>[2x]MRGSHHHHHHGSGTDITNQLTNVTVGIDSGTTVYPHQAGYVKLNYGFSVPNSAVKGDTFKITVPKELNLNGVTSTAKVPPIMAGDQVLANGVIDSDGNVIYTFTDYVNTKCDVKATLTMPAYIDPENVKKTGNVTLATGIGSTTANKTVLVDYEKYGKFYNLSIKGTIDQIDKTN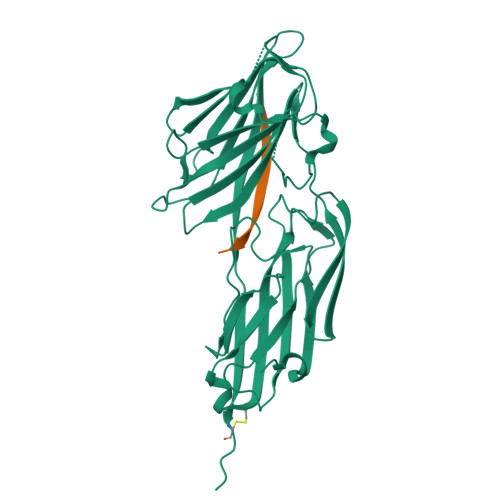NTYRQTIYVNPSGDNVIAPVLTGNLKPNTDSNALIDQQNTSIKVYKVDNAADLSESYFVNPENFEDVTNSVNITFPNPNQYKVEFNTPDDQITTPYIVVVNGHIDPNSKGDLALRSTLYGYNSNIIWRSMSWDNEVAFNNGSGSGDGIDCPVVP;>[2x]QHHLGGAKQAGAV> MSKPWLFTVHGTGQPDPLGPGLPADTARDVLDIYRWQPIGNYPAAAFPMWPSVEKGVAELILQIELKLDADPYADFAMAGYSQGAIVVGQVLKHHILPPTGRLHRFLHRLKKVIFWGNPMRQKGFAHSDEWIHPVAAPDTLGILEDRLENLEQYGFEVRDYAHDGDMYASIKEDDLHEY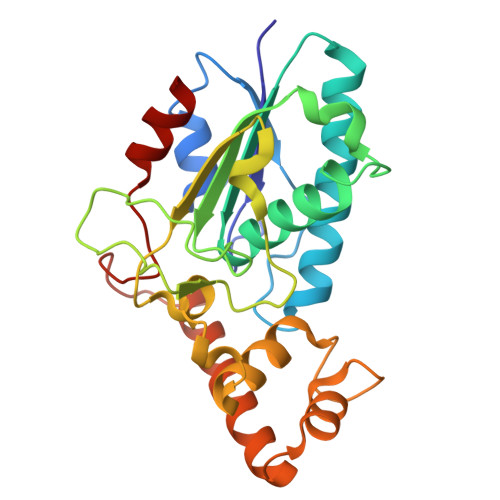EVAIGRIVMKASGFIGGRDSVVAQLIELGQRPITEGIALAGAIIDALTFFARSRMGDKWPHLYNRYPAVEFLRQI> KKVCACPKILKPVCGSDGRTYANSCIARCNGVSIKSEGSCPTGILN;> IVGGYTCAANSIPYQVSLNSGSHFCGGSLINSQWVVSAAHCYKS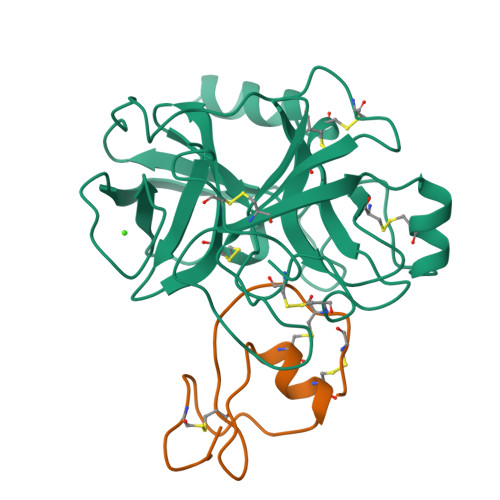RIQVRLGEHNIDVLEGNEQFINAAKIITHPNFNGNTLDNDIMLIKLSSPATLNSRVATVSLPRSCAAAGTECLISGWGNTKSSGSSYPSLLQCLKAPVLSDSSCKSSYPGQITGNMICVGFLEGGKDSCQGDSGGPVVCNGQLQGIVSWGYGCAQKNKPGVYTKVCNYVNWIQQTIAAN> SVAKTGMRDITALELTKDMRLGWSLGNTMDAYYSAASGLATETCWGNPKTTKA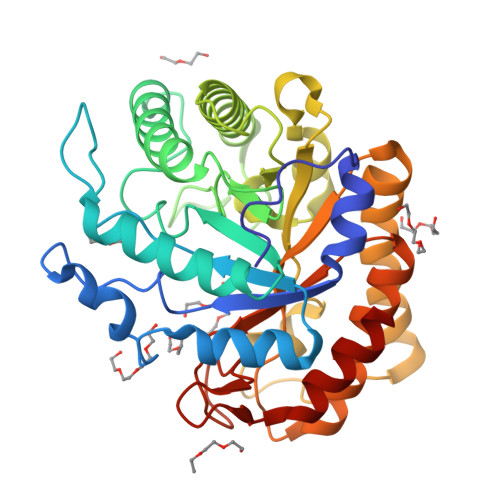MIDKVKEAGFNTVRIPITWAGHFGSAPNYTIDSAWLSRVEEIVNYVLDNDMYAIINLHHEENTWLVPTYANQEVATAQITKLWEQIATRFKDYSDYLIFEAMNEPRVVGGSAEWTGGTAENRAVINSLSLAAVNTIRATGGNNEKRFLMVPTHAACSLTDAVNDLVIPNNDSKIIVSLHMYSPYYFAMVSNSTPTWGTDSDKSSLSYELDAVYNKFIKNGRAVVIGEFGSIDKSNLSSRVTHAQYYAQEATKRGIPVCWWDNGYYGPGKDNSYALLNRSSLTWYYPEIVQALVKGSGYTV>MSATSTATSTSASQLHLNSTPVTHCLSDIVKKEDWSDFKFAPIRESTVSRAMTSRYFKDLDKFAVSDVIIVGAGSSGLSAAYVIAKNRPDLKVCIIESSVAPGGGSWLGGQLFSAMVMRKPAHLFLQELEIPYEDEGDYVVVKHAALFISTVLSKVLQLPNVKLFNATCVEDLVTRPPTEKGEVTVAGVVTNWTLVTQAHGTQCSMDPNVIELAGYKNDGTRDLSQKHGVILSTTGHDGPFGAFCAKRIVDIDQNQKLGGMKGLDMNHAEHDVVIHSGAYAGVDNMYFAGMEVAE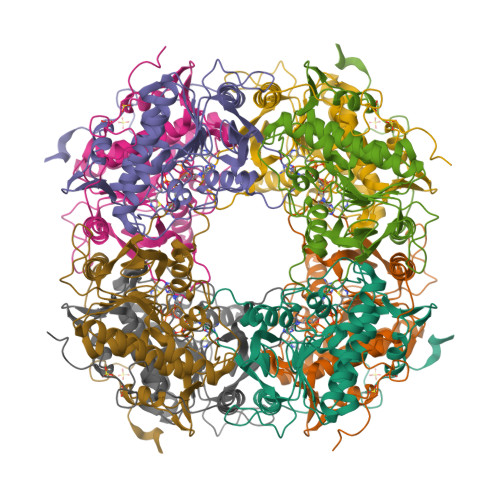LDGLNRMGPTFGAMALSGVHAAEQILKHFAA[2x]> MAHHHHHHVDDDDKMVHHDGFQTVKATIDWEHPMFKLYEKAKRNGKWNPADIDFSQDQKDFASLTSEEKISALPLVAGFSALEEAVTLDILPMAHALARQGRLEDVLFLTTFMHDEAKHVEMFSRWQQAVGIGQMDLSVFHNDHYKRIFYEALPEAMNRLYADDSPEAVIRAATVYNMIVEGTLAESGYYTFRQIYKKAGLF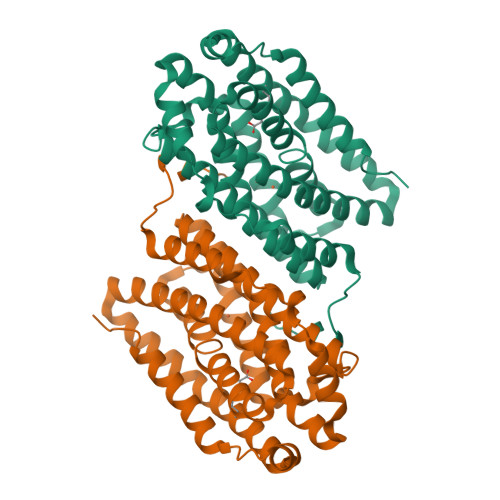PGLLQGIDYLNMDEGRHIQFGIYTIQRIVNEDERYYELFIRYMDELWPHVIGYVDYLTELGKRQQQLARTYALEIDYDLLRHYVIKQFNLRKKQISRTKRVDVVEGLEKTAAES> APLDLNNIQGDILGGLPKKTETYFFFKITDAAAFRKHLKQLIPLITTTAQVQKDRKAIDEHKKSNQKSGKPPELLPLAGVNIAFSHAGLKKLGINDDNLGDTAFKAGQLADAQNLGDPGTGNAGAKFVPDWDPAFKEKDIHGVILVAGDSHETVDKKLQEIEAIFGVGGPHASIHEVLTIQGDVRPGDEKGHEHFGFQDGISQPAVKGFDTNPNPGQAPVRPGVILVGRDGDSVANNARPSWAKDGSFLVFRKLQQLVPEFNKFLEENPIKLPGNNLTPEEGSELLGARLVGRWKSGAPIDITPLQDDPELAKDPQRNNNFRFDHPFADEQDSQTRCPFAAHIRKTNPRADLEDASPTSVESRRIIRRGIPYGPEVTPEEKESKKTKHDRGLLFVCYQSNIENGFQFIQKSWANNPNFPPSKPNPVTPGFDPIIGQAANNDGARTMSGTDPNNQANELSLPTELFVVPRGGEYF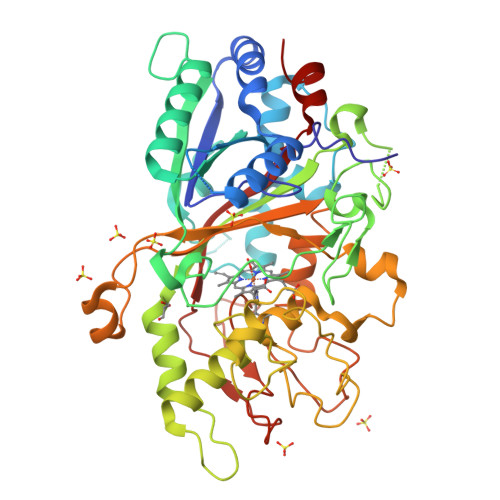FSPSISALKDTFAA>MKQSEFRRWLESQGVDVANGSNHLKLRFHGRRSVMPRHPCDEIKEPLRKAILKQLGLS[2x];>[2x]MRYPVTLTPAPEGGYMVSFVDIPEALTQGETVAEAMEAAKDALLTAFDFYFEDNELIPLPSPLNSHDHFIEVPLSVASKV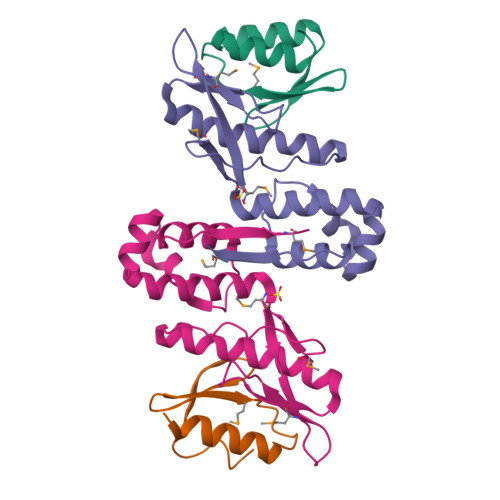LLLNAFLQSEITQQELARRIGKPKQEITRLFNLHHATKIDAVQLAAKALGKELSLVMV>MRDKELKFLVVDDFSTMRRIVRNLLKELGFNNVEEAEDGVDALNKLQAGGYGFVISDWNMPNMDGLELLKT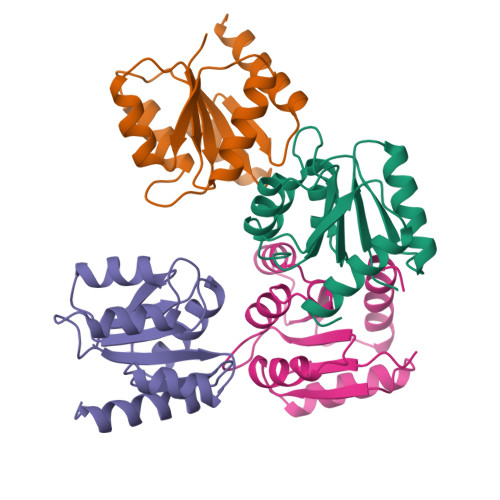IRADGAMSALPVLMVTAEADAENIKALAQAGASGYVVKPFTAATLEEKLNKIFEKLGM[4x]>[2x]APQQINDIVHRTITPLIEQQKIPGMAVAVIYQGKPYYFTWGY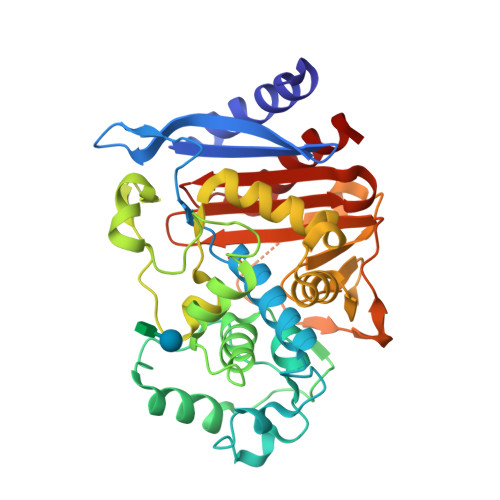ADIAKKQPVTQQTLFELGSVSKTFTGVLGGDAIARGEIKLSDPTTKYWPELTAKQWNGITLLHLATYTAGGLPLQVPDEVKSSSDLLRFYQNWQPAWAPGTQRLYANSSIGLFGALAVKPSGLSFEQAMQTRVFQPLKLNHTWINVPPAEEKNYAWGYREGKAVHVSPGALDAEAGGVKSTIEDMARWVQSNLKPLDINEKTLQQGIQLAQSRYWQTGDMYQGLGWEMLDWPVNPDSIINGSDNKIALAARPVKAITPPTPAVRASWVHKTGATGGFGSYVAFIPEKELGIVMLANKNYPNPARVDAAWQILNALQ> MGSPKNYIEMKPHPWFFGKIPRAKAEEMLSKQRHDGAFLIRESESAPGDFSLSVKFGNDVQHFKVLRDGAGKYFLWVVKFNSLNELVDYHRSTSVSRNQQIFLRDIEQVPQQPT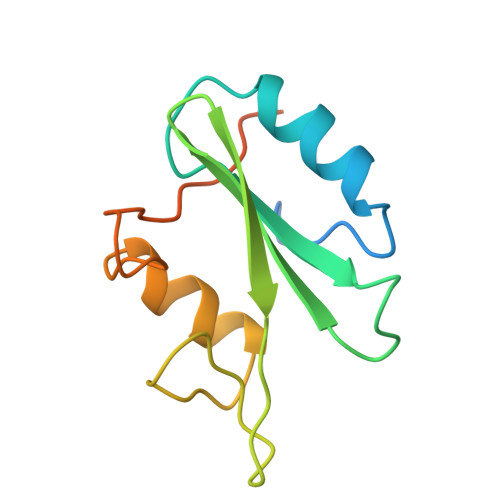YVQALFDFD> AQTVPYGIPLIKADKVQAQGFKGANVKVAVLDTGIQASHPDLNVV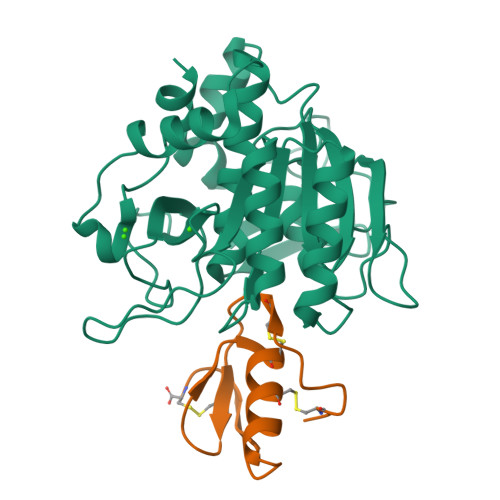GGASFVAGEAYNTDGNGHGTHVAGTVAALDNTTGVLGVAPSVSLYAVKVLNSSGSGSYSGIVSGIEWATTNGMDVINMSLGGASGSTAMKQAVDNAYARGVVVVAAAGNSGNSGSTNTIGYPAKYDSVIAVGAVDSNSNRASFSSVGAELEVMAPGAGVYSTYPTNTYATLNGTSMASPHVAGAAALILSKHPNLSASQVRNRLSSTATYLGSSFYYGKGLINVEAAAQ;> VDCSEYPKPACTLEYRPLCGSDNKTYGNKCNFCNAVVESNGTLTLSHFGKC>[2x]CA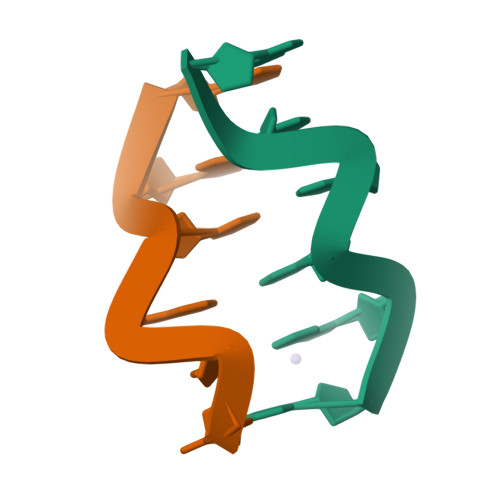CGCG;>CGCGTG[2x]>[2x]MGQQPGKVLGDQRRPSLPALHFIKGAGKRDSSRHGGPHCNVFVEHEALQRPVASDFEPQGLSEAARWNSKENLLAGPSENDPNLFVALYDFVASGDNTLSITKGEKLRVLGYNHNGEWCEAQTKNGQGWVPSNYITPVNSLEKHSWYHGPVSRNAAEYLLSSGINGSFLVRESESSPGQRSISLRYEGRVYHYRINTASDGKLYVSSESRFNTLAELVHHHSTVADGLITTLHYPAPKRNKPTVYGVSPNYDKWEMERTDITMKHKLGGGQYGEVYEGVWKKYSLTVAVKTLKEDTMEVEEFLKEAAVMKEIKHPNLVQLLGVCTREPPFYIITEFMTYGNLLDYLRECNRQEVNAVVLLYMATQISSAMEYLEKKNFIHRNLAARNCLVGENHLVKVADFGLSRLMTGDTYTAHAGAKFPIKWTAPESLAYNKFSIKSDVWAFGVLLWEIATYGMSPYPGIDLSQVYELLEKDYRMERPEGCPEKVYELMRACWQWN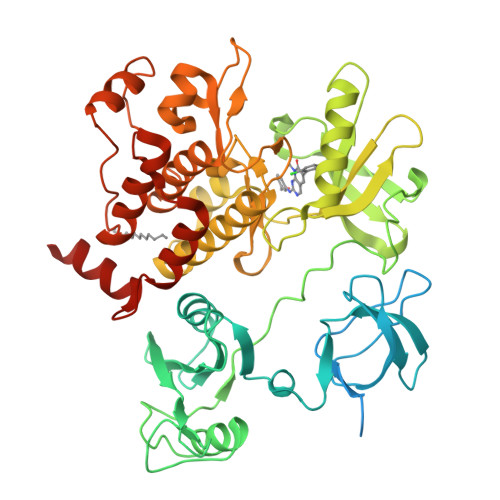PSDRPSFAEIHQAFETMFQESSISDEVEKELGKENLYFQ>MKKENQTQEIEERYQALFSNAAAVKALTQVVANSLGPKGLDAMLVDRFGEVVVTNDGVTILTLMDAQHPAARMVVNMARAQEREVGDGTTTAAVLAGALVSEGVNQILKGVPVSKVLAGMNRALNHALFLIRKNAIKVGSITDDRLLAAAKIAGRGDERVAAILRDAAAMLEDKLQDPGFKLADLVLAKVGADTTLIPGVVINKSPLWEEGSQKLQEVRLLVLDDGLYPEEVEEEALASEAGFEQYLKNQKIFQENLKKLKELGVKLILLTRGISDIAEEFCYENEIMVITRITQKELKRVLEFTGARAAKRTSLNKPVEELQKMLGYARTCFYDSRLDFTIIEGGAGKATATVLIGAATDEVVDEQERIAKDAAGSFAAAYRSGVLPGGGAFFLYLSREVESLKNRLPGMESYGVMAFSEALKVPFRVMAENAGFNGLEKLGDLMTLQVQKNNYALGLDFETGEFIDMIAGGVVDPAEVVYQAVKNASEVAISLLKINTIIKMKDYEVLKEGEQEDGGKR[4x]

Here we describe the prototype crystal structures of the bacterial Group III CPN from Carboxydothermus hydrogenoformans (Ch-CPN), an extremely thermophilic, carbon monoxide utilizing bacterium isolated from a hot spring in Eastern Russia. The subunits of Ch-CPN assume the modular structure consisting of an equatorial domain, an intermediate domain, and an apical domain. Like Group II CPNs, Ch-CPN is a hexadecamer consisting of a doublet of octameric rings, its subunits interact between the rings in a direct rather than staggered subunit to subunit fashion, and achieve cavity closure independent of co-chaperones. The closed state with a non-hydrolyzable ATP analog and the open state with ADP represent the conformational states of Ch-CPN before and after ATP hydrolysis, respectively.

The crystal structure of the ADP-bound Ch-CPN shows its fully open conformation. Eight subunits are combined to form a short cylinder with inter-subunit interactions mediated only by the equatorial domains. The stem loop of the S1 equatorial domain is associated with the C-terminal strand of the S2 equatorial domain to form an inter-subunit β-sheet, which contrasts with the corresponding four-stranded inter-subunit β-sheet in the closed Ch-CPN. The N-terminal residues 9–13, a β-strand in the closed Ch-CPN, assume a helical conformation in the open Ch-CPN, explaining the disparity in the number of strands between the closed and open states. Two short cylinders are stacked to form a long cylinder with ~ 85 Å in height and ~ 160 Å in width. Although ADP is bound to the AMPPNP binding site, it lacks interactions with Ile152, Arg155, and Asp373 of the intermediate domain, and Asn55 and Asp56 in the stem loop compared to AMPPNP. In addition, no magnesium ion is observed despite the presence of MgCl2 in the mother liquor. Although the binding mode of the adenosine of ADP is nearly identical to that of AMPPNP, the diphosphate moiety of ADP assumes a different conformation, which in turn gives rise to different interactions. Overall, the loose binding of ADP, the product of ATP hydrolysis, facilitates the product (ADP) release to vacate the site during ATP binding, initiating a new cycle of protein folding activity. Notably, the β-sheet is the only inter-subunit contact in the open conformation, indicating that it is responsible for allosteric communication among subunits at the onset of ring closure.> KYSKRIAWMKTTICDSLQLKDMIVEESFQYEKNKNLLEQFLSGEGLNKIFAYYQVQEQAQNDDIKDTGAQDPVLFFTTGDLEKIQDKAVWFLRITNPADDKKKASQQDGNDNDIIFGEITPNTVPMLNALMESVYSRQIDHIITEKIQFWGVAEEEQVLEFQQHSNKFSSEVREAINLMSPGTEHFKLDYEAISGLSESEKMQHYEMKFNEWINLISSQLNDDSEVRKDEKDAGPATELIYWRSRMQKITNWSEQLKSKDFQIVKASLQRHKNHDNQRPRGDESLSKLMMEYNRLDLLLTDKLNEAKDNVKYLTTLEKFIEPLYNGTPQQIIDTLPALMNAIKMIHTIARFYNTTDKMTGLFIKITNQMIKNCKDRILNKKDNGDNPSLYKMIWEQDPAELIEVLGSCIKLYCEYKKCYNDTKEKVADMPKGKTFDFSDAQIFGKFDTFVRRLQKLIEIFSNIQQFNALAKHNLEGMDVLTNKFKKIIDDFKKKGHNLLDTANNKFDRDWVEFNVEISHLDGELQNFIDNNFNRFRNIEYSLKLLHKFQSTIKRDSLKHNLTSRYNAILHNYATELDTIQRVFQDQKSNPPLVRNMPPEAGKIIWARHLFQKITGPINIFPENVINSTEIRRYYGSYNTLGKQLTIYEMWFYQDWVNKIEQSKAALQATLIVRHDENKKLYVNFDLEIMQLIREAKCLDRQGIEIPESARIILLQEDKFKTYYNELLYALKEYERINSKIKPICKNLLLPHIEDLDLKLRPGMVTLTWTSMNIESYLYYVHQGLKKLEQLIINVNDIIENRIENNLKTVSKVVLVHLPQDTKPLSLDSFVQLQEEYINSKTDFLTSKNVEVERAVDDLLQTIMLYPLDPHVDPVLPEETKRIKRYYFWYFYQALLNSTQNSLNAMKYRVCGKKIPGANTLQNLKPFFQVEVQLNGDKVTLNPSLQEIQKSINRAATAVLRCSKHLYNWDQQNKDSTDKATFYDMIACDKEIVKVILLLTGSIQGTKNKVNEFLSGFTKFEWLCKESIQESIKKFSKNGPTLQNYEDQLKKFSQIEEEIEKIVPTYKIGAMELMTHNICTSLSTWAKEWKLQYSQDLHKRARQLLDSLTEQTKMLSTKLSKPVKDIDSLGYVMETLEQIRKEQAEIDMKFNPVQEMYSLLDNYLPGGITDKDEMDARSLLRRNWDILIQQAEIKGKEYQHKQAIYLKELKQSIKDFTNQVSIFRRDYEKNGPMVEGISPAEAMERLRRFEDEYDVKYQMYKINARGENLFGLQNQKYPELEKTDAEIKNLNKLYNLYDSVIKNIQQFKEKSWQDVSKDDLAKMEEDAGKYGEQCSRLPKDLKEWQAYRDLKNYIDSLREQLPLIISLKKPSIMPRHWEKIKEITNTKLNYENPDQFYIEEIMGAKLLDFREDIEDITESADKQLKIRTGLDEINLYWNDMQFQFGIWGKRDVPCMLNGLIVGTILERLEEDQLQLSTFNSQRHVTPFKAEVENLIRTFSDVNDTLDMWVKVQKLWTSLEPVFTGGDIARQMPLQAKQFQGIDKNWMKIMEKAVETKKVIPCCQNDMLKDFLPDLNRKLEDCQKMLEAYLEGKRKKFPRFYFVSNPTLLKILSQGSEPTSIQEDFEKLFDAITKVTFESAKDKKNPALKQITQIQQVIGRNEENISLTGYYVKCEGNIEDWLKKLEQNMQQTLKDIASAAAQQVFQVGLKEFVSSQASQIALLGLQILWTSKVNEGLERLSRNERNAMDIKRNEIKEHMNILSSMCLEDLNGAVERTKVETLVTIQVHQKDISMDLKCKDVNDFEWQKQTRIAWKTDIDECIISITDWDSPYSYEFLGAKERLCITPLTDRCYITLAQAMSMYYGGAPAGPAGTGKTETVKDLGRTLGVFVVVTNCSDQHRYRDMAKIFKGLVQSGLWGCFDEFNRIDLEVLSVVAMQVESITTARKQHMKKFMFPEEEIEIELIPTVSYFITMNPGYAGRQELPENLKVLFRGVSMMVPDREIIIKVKLASVGYLQIDLLAKKFNVLYRLCEEQLSKQRHYDFGLRNILSVLRTAGNTKRQEIKSDEEMLLMRSLRDMNLSKLVADDIPLFNGLLADIFPKLKEVPKKLYPDVEKKIPEEINAESYLINTPSFQLKIIQLYETCLVRHGFMLVGPTGSGKSTIMKILTEVLTKLGSPHKIVIMNPKAITAEQMYGVKSEISDDWIPGVFSTIWAKSNNRALKHTTWITCDGPVDAIWIENLNTVLDDNKILTLANGERIAMTENCKVVFEVENLNNASPATVSRCGQVYVSPTDLGYEAVIEGWIRNRKASGRAEESDKLGNILRKYLINMRFIELQSKECKEPMMDTSPVISVINILNLLTGCLQYFVQTQRTLSEQEYEKFIVYSMAWAIGGIYEAQDRVRFHELLLAKNAPIPQKGKENETVFDYYVSQDYLDWKICSPEEWVPPQSLQFSQLLLPTLDSFRAEMLLNFILTQPKSHTCSNSALLIGGSGTAKTSSVLLYCNKFDPQKMLFKRTNFSSATSPFMFQSTIEAECDFKVGKEFAPPGNKMMTIFIDDMSMPFVNKWGDQITLELVRQLIETGGFYMLDKTQRGNQRKMKNLQYIGAMNHPGGGRNDIPNRLKRQFFIFNMILPLSIEGIYGPIIKHMFKQKYFSDSTYKVIESLTSATIALWNKVKSTMLPTPAKFHYVFNMRELSRIFKGILTCKKDTINDAPKSMKIKPELFLVGLWRHEAERVLADKLVNNKDKDTVMGYIQEVSLESFSQIENEILEKYSSEKTFLFCDFLRPDVINEDGIIEEEAPKIYEAIDSLTELRKRCNFLLSFYNDRNPSKKMPLVLFDDALKHLLRISRIIRQPRSSGLLVGVGGSGKQSLTRLAGFIGKNLIQQIIVTKTYSDKDLKEDIKKGFDDAGHLGKQVTFLMTDSEVKKEEFLEYINMVLSTGEIPNLLAKDEREVWLGDISQAYCKEKNLGNIDPPQSELWTYFVDRVRDNFHIMLCFSPVGQKFRERARKFPALFNECTIDWFLPWPEEALVSVAETFIKNFDKLDTKEETKQELMKHMGNVHLMVNEICDEYYQKMRRQVYVTPKSFLSYLNSYKTLYIEKYDELDQQEESFKIGLNKIQEATITINQMEISLKEEEIQLNEATEKTNQLLANLDKESKKANQKGEEVAATNKQCEIQAEQISKEKEEAERELEAALPALRRAQEAVDSIESKDIVELKANKKPLDIIKYIMDAVLVFFKARLIPIQIEERVFNKKEGKAVLFLKESYDESGIQTLGDMNFMKKLKEFEKDSINEETIELLEPYLNQSEDWFNDTFATKASKAAAGILKWAFAIYEYHQKSKIVKPKRIQVAIAEGRQAIALKELEKAREDLAQIQAYIKNLKDVYTKQMEEKNELEMKAAKTKKKINTARTLITSLSGEKDRWGKGAQDISDQKRKLVGNVSLSTAFISYCGPFNAEYRNKLAQQRFVVDMKKRGVPVTPGLELTSFLIDDATIGEWNLQGLPKDDLSIQNGIMVTNSARYPLFIDPQGQGQNWIRNKLSASIIPERCITTLSHPKFKDMFLKYCMESGLTLIVENIENEVDPMMDPVLERQIIVKGKTQFVNVAGTEMELSKEFKLFMTCRLANPSFSPELSAKTTIIDFTVTQSGLEQQLLGKVISKEQKALEDSLNQLLADVNQNQKDLQRLDKNLLERLINSQGNLLDDTELMDVLNNTKTQAKEVAAKLIDAEIKTKEINEKREQYRPVAIRGSAIYFTMIEVSLVNWMYNSSLEQFLKLFIESIDLSEKAQLPSNRVKNIISFLTFHVYRYVNRGLFEKDKITFILMMAFKILTTAGTISSGDVSLFLKSGDALDIKSERQKQISYLEDNQWLNILALSKHTFSGQTLPFFKELPDLISRSENQWRNWIDKNDPENFPIPDFAESINQEKEIGSFISLCLVRSLRNDRTLIATQNFISNVLGKEFTDPISYPIEGIWQESSNMDPVLFLLSAGADPTSSIDELAKKKKKFPCEKVSMGEGQERVARQVIMKGFVEGGWVILQNCHLGLKFMEEIETLVSPINQIHEDFRLWITCEQHPKFPLGLLQKTLKVTNEPPKGLKAGLYKTFTTIITQEFIDKVDHSNWRSLIFTICFLHSIVIERKKFGPLGWCVPYEYNYSDLEASLLYIEKYLTNLMSTPQPNSHNLPISMNVVRYMICEVQYGGRITDDLDRELFITYGETYLKDGIFGNDYFFYDIMVDGSGQKFKYRIPQNPSAELIKYQEYIAKVPTVDNPEVFGLHSNADLTFRLKESKEMINTVMETRPKDSSVGGGKTREEIVQDKAKDMLKNLPPDYNDVEVRELVSKLGGPNPKTSTERGMTVPLNIFLYQEVTRMQRVIGLVRKTLQDTILAIDGQIIMTPEILEAINAIYDAKVPNSWLYDPSGAEISWLLPNLGSWSTSLSDRNKQLNDWLRSGQRPILFWLTGFFNPQGFLTGMKQEVTRNHKKGDGKGGEAWSLDDVVYSTTVKEREKEKDIEQPPAEGVYIKGLYLEGCKWSKNGLDDSDPKKIFADLPILHVSAINKKKTNEQDRMSNTYLCPVYKYPKRTDKYLIFRVGLPCEGSNNPSHWKLRGVALLCST;> MGDHSQKDSPEDFIINRLSQALGIQKEKIKKSLETQQDDKGEVTNKDEFQGFIQQDNSTNILWVSGQSEKCTFYYGQLPPIDKFKKKGIAVIKLGLHKLTNENVAKDVVVVEITNNLLEHLNSVFNEIMSPVMQNPLNQQGWTDLVAKDLMEKFNNYVAQVYVLLGQIKGKTMLPLPSHKLTSSDTTPDKDKAHVFEGSIITWTKQIKNVLKLEPEQLLKYGNDPGPLAEIEFWQNKRDNLNLIDSQLKSVEVQNILHFLDNNKSTYTTPFTKLQAEVKKARLEANENYRYLFTLKDLFSKLQESQPSDFPTLYELFIPIMHTILLIYNKSKTYNQPPRLVVLIREICNAIISNAQAFVDKDTIFSLIDSKETTEACDKLQVTLDVCSKFKDAYFEYKAKAGGNWKLTSNALFVRLDSFLERCQDILHLTNTIVQFNKLEKIELGGTKGKTLTESIAQIFKEFEEAVQAFTSVSYDIMNIAEKKFDDDFYEFRSKIKELERRLASVITQGFDDYDTIYGRFKLLDNFEGLLTRPIIADELEKKHIVLLEMYKQDLKQVQSIFLEGKQFVDSMHENAPLFLNMPPIAGALTWCKSLRDRIQEPIEKLAQLGQGITEREEYKDVQKLYTSITKSIKDYEDQKILSWEKEVEDSSQDKLKQTLLCKDENDLIKVNFDPSLVRLLKEVKYFLLLRLEVPTTAKDIYTKAETYRTQIVALDMIVDNYNHIKTCLLPVEEPLVKKKIQDMEEEVKPGIEEIRWKSTNIDQFISKSKSIVDQLFETVNKMKDSLQKIHKSLANFNVKIIERKNRPMSPDDYDQFLKAIFSNKLTIVKDNGNQIQKLVKEVLDAVKADKKQNSWKNYNDYVNVIVIEGISTAIQTALLHLNEQINPVFIKRNDISPLFDIRLELGQSGIQFDPEIGESSNQLTVRNTIRNWINDFFNIAGTIQRLDTTMPGDFLQEIRSFFEIKQCLAMITQNLEWIENECNQFRARFDTYSYLWTEDEQISFNRFLDENEPKDEDGKGGDDDEGENTEKQNPLLKGCRAKIPNLDLFDEKITHLKAIQQEISRIKTPEDISWLRINLQPMKTALDARVTRWIRVYTDFLVNQFRTTQKNLLDFIEKTKDGIKKNPADHENLHDKKLLMSVMKVISDVKDVEPRREGIITRMKEMVTKLKKHNVPITEKGTDDPLQQIDNANSNFIEIYGRVFKVKADIIPLQAEETQNIKRDLDIFMKEVESFRKEFMQKLPFDYTESMGYENINNAYDTIMVYYHKLTAIEGRALEYNNLEKLFELQKSNYKQLKDCMNDLKNLKTMWDAIALIHFQYNDWKTKPWRQIKADILLDTNKTLGTQIKNLPKEIRNFKGYNVIVEKVKNMGTVLPLVSALHSEFMEDRHWSQLKQITGTVFDHNSLSFYFEDILALNLYKYENTVNEIVDVAQKEAKIEKKLKNIEQWWSKQVFEFTEYKETKTFASLDNMMEVLDQHSLDLMGMKSQGKYVEFFYDRVEDWREKLGRVDVVVNEWLKVQKNWKILYNIFLLSEDIRMQLPEDTKVFEGVDKEFKDMMSEVSANPSVVEACTIERRDVLVGWSQAIKKCEKALNDYLEQKKKSFPRFYFLSNQSLLTILSNGQNAPKVCEYLGDCFDGLKTLTFEPPANPAETSKVGIGMISKDDEKVPFSSKFICEGAVEHWLLNLEFRMRETLQEILEGAKNTADLWDSGDKPREEWVEGYNAQIALLTTTIVWTEDVGRAFEDLAGGSETAMKECQKLIEVRLENLIKKVRGDLHILERWKIINIITIDVHSRDVVEKFVIQKVSEAESFAWLSQLKFYWENKPDSDMHLRQTLRFPWEKDKNKNKCIIRIVDWFRFYSYEYIGNAIRLVITPLTDRCYITLTQALNLTMGGAPAGPAGTGKTETTKDLGRAIGIPVMVFNCSDQMNKDSMAQIFMGLSQSGAWGCFDEFNRISIEVLSVVSTQVKCVLDALKEKKTKFSFVEEGEIQLQDTVGFFITMNPGYAGRTELPENLKALFRSCAMVVPDLALICENMLMSEGFTMARVLSRKFVSLYMLSRELLSKQKHYDWGLRAVKSVLRQAGKLKRGDPDMPEDPLLMRALRDFNMPKIVTDDKVIFRRLIGDLFPKLDPPTKQNPELKKIVQDTTKKDMGLVAEELFVTKVVQLAEILEVRHCCFVIGPPGSGKTCVWKTLIKSYINSGEDAEYDTLNPKAVTSDELFGAYTKTKEWKNGVIAVIMKNQVKNEEKYKATHMHKWSVLDGDIDPEWIESLNTVMDDNKVLTLVSNDRIFLTPQMRLIFEISNLRNATPATVSRAGVLFINETDIGWMPYMNSWLERSQINILKQQKEMANMPEYPVIDDVAKSVFYRCFQSYFEQNIDVHDKNRVRHICPMVDIAMIQTICTILDALLIQHLPKLKQMKEEDEKQALEAFFIFAGLWAIGGPVGGGQDDSKDMKEFNTVWKGAAKVKFPEQGLCYDYYYDINENKWNTWKVEDYLPNDQPLFSKIYVATIHTTRLRYMIDIHLQRRKPILFIGSAGTGKTAVVRDYLNSTRPEQVSHKTINFSSFTDSLALQKNIESMVEKKNGRNYGSATNKVLICFIDDFNMPYVDKYGTQSPIQLLRLILDYGSIFNREQLEERKFLQDLLFFGCLNQKSGSFTVDLRLQRNFSVFSMYTPSSDVIKTIFGSILNAHLSTIDDKAQKMAFKLVEATYFTFDKILKNTTAFAPSAKRFHYQFNFRELARVCEGICRTTPGQYSGGDQGKLVRLWAHEMKRTFEDRFIANEHVEFFRRYLTEAISKCIGEFPETENPIAEPLIFTGFVAAHQGLDQQYTQCTIPVLKRVLDDKLEEYNEVKAQMNLVLFQQAMEHVSRICRILDMPGNNALLVGVGGSGKQSLCRLSTFINGFEIDQLVVTASFTINDLRNNLQEIYKKIAKPNSIARVFMITDSQIKEEQFLIPINDMLNSGWIFDLFPKEDMDSLVSGVRNEAKGEGVDVNNLTALTSYFLDKIRKNLKVVLCFSPVGDTMRIRSRKFPGIINNTSIDWFHPWPHEALIDVAFRFLEEIEFPTEEIRQSISLNMAKVHSSIDTANEKFLKLERRYNYTTPKSFLELIDFYKKLLTEKRETIQRQIQRYEMGLNILAETQNKVQGLQEELKVKMVEVNKQREETDILIEKVGKESALAEEEQTIANAEEEKTNVAAAEAEKISKEATEALAEALPALRSAEAAVDCLKKPHVTEMKNLGSPPAGVIVTARVVLILFNQGITLNDPDEKVWKKAVTFMNNPQAFIDKVKSFDGENIEPNIIEQSNKIIQDPSKKFNEKDMAGQSYAASKLCAWAVNIVTFNKIFKQVKPLQDAQKQANEILEEKKKELAIVKQRVAELNARVNSLKRQLEEAEARKMIVEQDAARCQSRLSAAENLVNGLAGENKRWTQNVKFLKENIKSMIGDSLLASAFVSYIGAFSAKLRLELWKNTWLPDIIEKGIPITEGIEPLKILTTEAIKSKWKNEGLPADPMSLENAAIITACARWPLIIDPQLQGSTWIRGKQGENLTTISLSQPKWLGALTSSISSGRAVLIEGIQQEIDATLDPLLQRAVKKNGNQLQLEIGGDPIDYDPNFKLFLMTKLINPHFRPEIAAQCTIINFIVTESGLEEQFIAMVVNIEKNELEMAKQDLVKKQNEYAVTLDKLESDLLQSLSEADPATILDNTELIQNLDKTKKTTIEITEQQQKAKVTEAEINIQREHYRVVAAEGSMLYFLVISLSVMDHMYQYSLESFITFFFKAINRTTVRDENRIPTLILNIRQTIYQWISRGLFEKHKLIFLTLIVFRLMQKKIIDVAYEVAEMDFLIKCPARPGVENTLDWLPNISWDQIQGLINLEEFRNFAHQLEKEAPNRFKDWYNELQPEDQKLPLDWKRLDSMPFKKLLVLRCLRPDRMTISLNNFIRAVLPQGDAFVEMDQKLAFSEILESVINEDSESTIPIFFILSPGSDPVKEVEKIAKKKRIEPGKNFFNIALGQGQDEIARRRIEEGNKEGHWVMLQNIHLMPTWLIELEKILDSYSGEAGGGNSEFRLFLSAEPSTGIPIGILDRSIKLTNEPPAGLKANMKRAWTYFSKEEIEDKDPKIKSILFALCFFHSTLIERRRFGPKGWNMSYPFNMGDLRDSYLVMNRYMEQNQGGKVPFNDLIYIFGEIMYGGHIVDDWDRRLCNSYLFNTMHEQLFDELELFPYIEGKGLSFKVPGQNPYEKYIEHIETSLKQETPLAYGLHPNAEIGFRTDQCKTLFNTLLELMPKEQSRDEKSSDIKSSNEMASDLIKQLLEDSELKNKIFNMEEIKNKIDAENKGPYQNVFLQEIEYMNALLSEIVKDLEEIGQGLSGLLTVSENMEMIIESIALSRVPASWQKLAYPSKRGLQSWLANLFQRIEQLNIFRDDPYSIPRVVMISRFFNPQSFLTAIMQVISRAKAYELNKLYIQTEITKRSIEEIEGAAKEGAYVYGFILEGARWDYQLGQLEESKPKEMFSVLPVTYCKAIPLPPEGKEDKSLYQCPVYKTEDRGNTYVFTAQLKTRFPPRKWILAGVAIIMDVEGVSD;> PLVWTQLKQTGTTQPTARSGHTIITVGKTHIMFGGLDNDKNNYKDGKIAPNNQVFTLKLTQNNCEWRQIACQGDVPLPRCYHASCAISADKMLVFGGSYTSNLRFNDTYILKTTSYQWSKPANQISGGEPKNAESKIGAPQPRYGHSATFFEGKVYIFGGHGGINYQRLAFNDLYVLETENFEWTRLEPKGNPPDPRGGHSAAMMANKPQLMIFGGWSFTSQYSNIMIYDIEKDEWVDPEIAHEIPKWNLSGIMAPSIPSWKYFIFGGSVGSFEEGGNRTNSRFVDDSFVLDIDTLSWSSINLEADETSKAVCKPRPRESASIFYDSGESRAIVFGGWANNWLNDLWALNVSTITGPIFSIKPALGPLTGKTKVLIEGDGFKDTQNISVKFSGGKLEKEVNGTFVNEKEISCETPTFDYPRSVEVTVCMNKGDYTITKSAFTYTKADKTIAYGPGLLTENLIGVQTTIVIQARNGSDEFVVTIRNPAKIKKEEEVKEGDKANTKNTIKEDEEEEGEDEEENKKKKEAEKNDLTGSAVMNYISKQLKDIQEFIENTKENIEIRNKNISELINVMINLEKVRVKNDDDVLTLDTVEEMLNFLKKKKDSDIKKCKKLQEEWKNLAKMAQAVKKDIQNPVKTESDKTKENIKKFEEITLKEYANSLKKESFYKTGVSESFKRIGEVKQKVDEFEVQLNQYEDFARIGSKKLMEQIRTDVSSVEKLWVRIEISEKTMDEYKKMKWGSINSMDMEDEIKKLRKALTDLRGIDKRSNAFIGITEELKKWATFLPLLGELKDPSMNSEDGRHWKKLKDLVKKEFDVSQELMLEIIWDLKLFDYKDGIEEITDQAKQELKMEKALKKIIDFWRDIEFELVQHKNTDIHTLKMSEENFETLEDHQLQINNMLLSKYVAYFEKEVEKWKYDLGSVYDVVQLLLEVQKTWSFLENLFEVKRELPNESAQFVGIDKDMKEIMQKGCDIKNCLKFCTIEGMLKRLENIQAQLKVCEKALNEFLDSKRRAFPRFYFVSVNDLLDILSNGNSPAKINRHMSKIFQAIDNLQLKEDSSGGRPTLKMISCVGTEEVDFSSPRLLQGKVESYLKDVIDTMIGTLKSVANSSFKNFQSMTRKEWLKSDPSQITLLVNNIIWSKAVEDCFLKLQSGDINAMKLFLDESIKQLTELIGMVQGDLSKPLRQKIMCLITIDTHSRDVVHRLINEHVRKAEEFQWQSQLKFYWVDNDAKIKIADARFVYNYEYLGNGPRLVITPLTDRIYVTATQALHLKMGCAPAGPAGTGKTETTKDLANALAKACYVFNCSSEMNYESMGNIYKGLASSGCWGCFDEFNRLLPEVLSVCSVQFKAVTDAIKQNVERFIIEGDEISLDPTCGVFITMNPGYLGRAELPEGLKALFRPITVVVPDLELICENMLMAEGFIEAKILAKKFVTLYMLCRDLLSKQLHYDWGLRAIKSVLVVAGGFKRSEPEIAEQALLMRALRDFNIPKIAFQDLYVFHGLLGDLFPGINIKPKKDLDFEKIITDVCIENKLDPDPEFVLKVVQLSELLAIRHCVFVMGPPGAGKSTTWKILAKAQDKTNKKTTLIDIDPKVVSTKDFYGYNLPSKEWKDGLFSKMLRSLAEQPDTNPKWICLDGDLDANWIESMNSVMDDNKILTLANNERIPLKPHMRALFEIRDLRFATPATVSRAGILYISDEVGYQWRSYVKSWIKQEFSQDQEMSKNLDTLFGKYVPDTLDHIKKHCRFLVPVSPISQVISICKSLQTLLKGDVKNLEYLFVYALIWAIGGALAEKDSIDYRKDFSTWWKGAWKTAVKFPSKGTIFDYYVDQSGDSSKFVEWSKRLENKEFDPQVETMGNITVNTIETLATTEFIKSYLMVKHPSLLIGNSGCGKTQLAKGILKEIVQAKPENYAYQLINFNYYTDSTYLQGQIEQTLEKKAGRQYGPPGKVQLIYFIDDLNMPQLDAYDTQTAIALLRQLADYGHFYDVSKLALKDIINTQVLAAMNPSAGSFFVNPRYQRHFWTISIPFPDNESLSLIYITFLNGHLKRFKSTIQEYSNIIVRASLMLHQAVTQNFRKTAINFHYEFNLRHMSNVFQGLLLSDPNKFTEPDKLIKLWIHECERTYGDRLVSTDNLKTYKENIFDIVKKSFSKFNFSRYFGNNPENLIYCNFIAGINSDRFYDQMPNNEMEKHISEALKEYNDNNAFMGLVLFEDAMKHVCRICRIVLPSSGHALLVGVGGSGKQSLSKLASFIMGYTTFSITISATYSMVDLRNDLQQLYFKCGPKEEGILFLFTEGQITNERFLVYINDLLSSGEIAELYTLDEKEAMINQVRAKVKGEGKPDTRENCWNWFIDQVKKNLHMAICFSPVGDMRRRARQFPALVNCTVIDWFQPWPYEALFNVAKSFLEPVDLGDDKVREAVVKFMPFSFTLVNDLGLKLLEQERRYAYTTPKSFLELISLFTNMLAQKRESLERNKERYETGLVKLKETAEQVAIIEVEVKEKQVEAEAKKKEADAFAEVVGREKDKVEKENSKATIEADKCGLIKQNVEAQKSSTQQDLDAAQPLVEQAKSALNSISKKDFQQAKSFASPPAGVPEVFAATIYLLAGYFNEAIEIDKNKKPKDVSWKSSLKLMKSPEEFMEKLLNFKDVVDANQVANVNIVKNQYLNMPSFTPEQMASKSAAAKGICSWVVNIVKYYDVIQDVEPKRKALKEATEQLEEATVKLNEVEEVVRKLNEELNKLKAENDKAIAERNAAISEAERCARRLNLAQRLVTALSSENERWGKSIIQLEDQLKLMVGDVLVASSFVSYSGPFNKKFRNIMINQNFMKFMKEHTIPMSPDPNPIKILTDESTIALWNKQKLPSDSVSIENGTILTNSARYPLMIDPQLQGITWIREKEKANNLKILRLGSKNINRDLELSIENGYSAIIENMNERIDAILMPIIARSFIKRGKNKIIKFAGKDLILHPNFKLFLHTKLSNPHYPPEIQAEAALINFTVTEAGLGDQLLSLVVARERPDLAKMKIELITQQNDFKIKLKDLEDELLYKLANAKGDILDDIELIENLEYSKKLSVEIAEKVAAAKITEAKINETSENYRPAASRGALFYFLLSDLSKVHSFYKYSLESFIVVINRAIDAISENKIYGKTTMMSPRSLKKRVDELIESLTYTAYQTTRRGLFESHKLIVAAMLCLRVLLRSEELNSDEVDHLIIGKVDVNPTPMPDALKSFLNDNIWAACKALETIHQFQGFCQSLETDVLQWKKWYSEEKAETADLPKAFKELSKFHRLLLLRALRPDRLPSALSQFVHDKMGERYIEQPPFNIFETFQETSKTVPIFFVLFPGVDPTPDVERVAATFDVSANNGRFINISMGQGQEDRAKKALFDCAQKGHWIMLQNVHLMQSWLYGLNGLEGFLESVFASPKTHPNFRVFISSEPPNVLLPLMQIIPESILQGSLKIANEAPQYLKANLRRAYNKFDQEFLDKCDKKPTEFKSCLFALCFFHSLMLGRKKFGTQGWSRVYNFNDGDLTICADVLYNYLSKYDQVPWDDLRYIFGEIMYGGHITDDWDRRTNRTYLKVLIRSELLQQNFNLAPQFKSPDPSKFDYEAYRKYIEEKLPIESPQMFGMHPNAEIGYLTQTCDQVFNTILEVQGGSSGGGASKKDDGVMVTLTDFKTRCPHDFNMLLIEEKVKEKTPYIVVCLQECERMNGLLKEIKTSLEDLRLGLTGALNMTDAMESLQQSLSFNKVPDTWEKKAYFSKKPLSSWFADLIERNIQLQEWCKELVTPTSLCISYLFNPMSYLTAIMQFTARAQGLPLDGITIQTNVTAMKGPEDVVNPAENGAYIHGLFLEGAAWEIGGQGQDGYLIEQKPKELHPKMPVINAVAVPLDKKKKNGQYDCPTYVTSARGQTFVFTANLNMESDDSDPNKWILSGTCMLMSDD;> LTAQELNEDMPSKMLEPKNPQAPKNITVYDYYTRKFKTDELVDQMIVHFSMDGDYIWKESNEYKTQEEIRDTKKALIKEAMRKQESEEPGANHDEEAIKQTLRNKFNYNTRECQTINPSIRERGVSTEPPPSDTICGNITQWEIFDAYYAEIMKDHQIENKKKKEVDQDKKQDQSMYSTSFKRCCKIMERMVVQNDQEDKYHDYRYYWSQGDNLEAGKNEGHLLPIWRFSNEKQRKKNVTSICWNPLYPDLFAVSLGSYDFTKQRMGLICLYSLKNTTHPEYAFNCEAGVMCLDFHPKSAALLAVGLYDGTVLVYDIRNKHKKPIYQSTVRNQKHTDPVWQVKWNPDTSKNYNFYSISSDGRVMNWILMKNKLEPEEVILLRLVGKNEEESTLIGLACGLCFDFNKFEPHIFLVGTEEGKIHKCSRAYSGQYQETYNGHLLAVYKVKWNNFHPRTFISASADWTVRIWDSKYTSQIICFDLSMMVVDAVWAPYSSTVFACATMDKVQVYDLNVDKLNKLAEQKIVKQPKLTNLSFNYKDPILLVGDSHGGVTLVKLSPNLCKSGPEIKQTEDKKAMEEFKNVKIEDYEREKMENL;> KEFNNPINFQDTETRYGGIQNQVVNINQYVQRNPNFIDLDNIAELSEHSVNTERVKTGDRGMSHKEGGWPGNVDPNEAQETGRFKKRIEKDTSFPQAVKDLKEGVEKCIYQNNQIDLLEEYFEGETSEHVVENLSSKTLMLFKDEKEICKRSVSEISWHPEGPTKVAVSYAIMRFQQMPEKMPTQAYVWDLLNPNSPEIKLMSPSAVTNISYNQKIPDQIGGGCYNGLLAVWDGRKGENPIMISPVENSHYEPVTHFHWLMSKTGSECVTTSTDGKVMWWDTRKFEAGPVEKLNIIEGLGENEEIIGGTALEYNVEAGPSKFLIGTESGSILTANKKLKKPVEITTRYGLDQGRHLGPVYSINRSNQNPKYFLSVGDWSCKIWVEDLKTPIIRTKYHGSYLSDGCWSPTRSGAFFLVRRDGWMDVWDYYYRQNEIAFSHKVSDSPLTCIKINQTGGAYHNSGKLCAIGDQDGTVTILELCDSLYTMQPKEKDIINEMFEREYRKEKNLETIKKQQELAKRQVQKDMGSQKEKWEKKKLEMIETAEASFHENLAKNPV;> NADDQLKQLSALEGANGYVIFNESGIPLKRHEKSISHEKAVHIAALVSDLWNVSKKVIQRDLKTPENDIEVIRLRTKHSYEYIITQSGDFTMLAIQLCGKAIEEAKKAAA;> MSEVEDTLNRIKTHKTVLGYLIVNSEGGVVRGAFKDEEESKNIANSIPLLTKKARSVVRDLDPTNDLVFLRIQTKLNEIMVAPDDEFSLIVIQTKG;> SHLDKVQPVIKNSDMSVEMQKEVEEVAKKAIDYCNTDKEIATFIKDDFRSRYHGTWHCIVGRNFGSFVTFERSYYIYLYVGQLAILLFKTG;> KAVTDMDINELRKLMIGKAIINSSDMQGDLLQEAQDVIQSGIENNSAPVLNIEAACKYIKENLDKKFGPTWQCIIGEGYAYDVTVQNNTLLFMFYNGNLAVLIFKS;> QQYKTFMGARVLWPPEAADDILEGAIRETQDALKKFEIAREGQKIAEHLKKYMDDHFDPYWHVFFGKNFGCQAVHNKNRFIYFYIEKTAFLMYQT;> HANEQIIDMPENSEMKSMKNDAFSQAKFAVENYKFENKISSHIKKFFDEKYGPNWHCVVGKHFNAYVSYDSKNFIFFYEGQLAILLYRKG;> EPLPPHIIRFNDMAQHLLKKVIRQADVLIKENPQGLEKDIALNLVKFVKSQPEFKIGDGEWQCIIGKNFGCSLTFDANVLAFFDLLPSRKSILLFKSG;> MNHEPEVKATDMEEDMIKRVKEIAINAVKEYKQEKQIAHYIKYEFDKIDGYGWNCIVGRNFGSHIIHQTKKYIFFKINELCLLLWKA;> TDKEYISEEVQKAIDDSVKQVFGIKDDSSQVTITYNKDKVNLWTQQIIDYTIRGLNKLGKHFKYCVTAILQQTNHAGISVQITAYQDTNTDGSLIQCYEINDIYAIVSVFAMAV;> RKREASLITLNYIKNRFYPSKIQKIIKELFEDRLKGVEYDPNNANQLSERLVLELREKIKRGKVPRYKIGVQVVFGEIKGQGLRIASKCLWDVQNDNYASYTYTSEKVYCTGIVFGCYFE;> TTTVTSEDHFMTFYNENNKKLIVVDVYPGWSGPCTAMYPTYNQLMISIDDFEKRIDILLLDQDKLVTYKNDKFHATCQPKFLFISEGKIIDEVLGTNIPVFIEKVNKYIPLS;> AKGTTCQKAIVNWEAANPGKNPSEAEEIKLIFQIPPIEKMDGPVLNTLTKCKKLSLSSNSIDKMISLNMLRNLEILSLSRNVIKKISGLEDIGGTLRQLWLSYNFIEKLDGLNNCSVLQTLYIGNNRIKNWEELDKLKDLPELENVLFYGNPIYEQVKEDPKLIVLKKLPTLKNVDGYIIDDSVLEKVKQIA

Thousands of outer-arm dyneins (OADs) are arrayed in the axoneme to drive a rhythmic ciliary beat. Each OAD is divided into two regions, a head that contains AAA+ rings (rings) for ATP hydrolysis and a tail that holds together the whole complex. The tail is permanently attached to the MTD A-tubule, while the head region of each HC contains a microtubule-binding domain (MTBD), which binds and releases the MTD B-tubule depending on the nucleotide states. We reconstituted the purified OADs onto MTDs to mimic native arrays and determined the structures, by cryo-EM, of free OAD and OAD arrays bound to MTDs (OAD-MTD) in two different microtubule-binding states.

Cryo-EM classification reveals that the OAD arrays adopt two distinct microtubule-binding states, MTBS-1 and MTBS-2. In both states, the relative axial positions for α- and γ-MTBD are fixed on MTD (γ-MTBD is always 8 nm ahead), while the β-MTBD position is equivalent to either α-MTBD in MTBS-1 or γ-MTBD in MTBS-2. The OAD unit together with the four binding protofilaments (OAD-PF) was locally refined to resolutions of ~2.8–3.8 Å for most structured regions in MTBS-1 and to resolutions of ~3.8–6 Å in MTBS-2. The arrayed OADs adopt a fully parallel conformation in which the three AAA+ rings are stacked together via linker–ring (LR) interactions. In MTBS-1, β-HC adopts a post-1 linker docking mode, which is precisely switched to post-2 along with β-MTBD stepping forward. On the other hand, α-linker fits well into a groove (groove-1) formed by AAA3S, AAA5E and β-CT-cap in MTBS-1, while β-linker matches another groove (groove-2) between γ-AAA2S and γ-AAA3S. In brief, γ-Ig-PT contacts β-AAA4L PS-I with the help of γ-kelch in MTBS-1, while the contact site is switched to the H2-β3 loop of β-AAA3L in MTBS-2. The TTH interfaces involve IC3, NDD and α/β-HB1–3 of the OAD0 tail region, and α/β-linkers, AAA2 small subunit of β-HC (β-AAA2S), β-AAA6S and the C-terminal cap of β-HC (β-CT-cap) of the OAD+1 head region. In post-1, OADs are attached to B-tubules and form ordered arrays. The TTH interactions between OAD0 and OAD+1 sterically restrain the nucleotide-induced allosteric response of OAD+1 and its downstream neighbors.> AIKSSILSFNSIITKNDEIKNEEAEFPKVLLFNDNYFDGNIYRINNALSGIEHDPMYYDLMCQSMKQQIEKIKIPLNSSETISVFAIAPQPLLLYLGYLLNDETNIKIYQRFRTGNLKWNWESSEITNNFYVEQLYTDGNEIDTEVNLILSLSAEISLDRIPTFSNQEYKVPTLILRSDRQGFDAIKSNEDVNEYISVFRNLVVEKIRNDFPNLKCINIFPATPVSVPVRMGMNYQKNIDVEWKIFNQQTNVGFIYSLSLKGEV

Here, we present the biochemical and structural characterization of two CBASS systems, composed of CdnG and Cap5, from Asticcacaulis sp. and Lactococcus lactis. We show that CdnG from Asticcacaulis sp. synthesizes 3′,2′-cGAMP in vitro, and 3′,2′-cGAMP is the biological signaling molecule that activates Cap5 for DNA degradation. Each monomer of Cap5 is composed of the N-terminal HNH domain, the C-terminal SAVED domain, and a short flexible linker connecting these two domains. The structures revealed that both Cap5 form homodimers, resulting from the side-by-side packing of two HNH domains.

To provide molecular insight into the ligand specificity of the SAVED domain of Cap5, we solved the crystal structure of the SAVED domain of LlCap5 (LlCap5-SAVED) in complex with 3′,2′-cGAMP. The structures of the SAVED domains of LlCap5-SAVED and the full-length LlCap5 are essentially the same (rmsd = 0.4 Å). In our structure, 3′,2′-cGAMP is found at the center of LlCap5-SAVED. Employing a similar evolutionary approach to describe the structure of LlCap5-SAVED, 3′,2′-cGAMP is bound at the interface of these two CARF-like motifs. Several conserved residues of LlCap5-SAVED are involved in the recognition of 3′,2′-cGAMP. Specifically, the adenine base is stacked between the side chains of I208 and R234, which is further stacked by the side chain of F304. The side chain of R234 also forms a hydrogen bond with the 2′−5′ phosphate linkage. The involvement of the side chain of R234 for both base-stacking and phosphate-hydrogen bonding appears to be only feasible with the 2′−5′ phosphate linkage, indicating R234 is the discriminating residue to distinguish 3′,2′-cGAMP from 3′,3′-cGAMP. In addition to R234, the side chain of S274 also hydrogen bonds with the 2′−5′ phosphate linkage, and the free 3′-OH group of the AMP moiety hydrogen bonds with the main-chain carbonyl group of T344. On the other hand, a single residue, R281, is responsible for the recognition of the guanine base.>MNAMANKYPTEQLKLWGKAKELREQYYMNYARAKEKGGIRWSGSAWALDAIPAGLGEDVYSLTGEPYAAAVAHDRKFAKECMDAAEAYGFARDLCSYMRIYWGGMHLNKYAFGGEFPKPDFVFQTQICCSHSKWYQHVAKEEKIPEFYLDVGVGPYRDMTDARLDYVANQLHDGIAFVEKASGRKFDDELFIKAVKNEMRSTSRWADICALNKVKPAPLDEKTMYSLYVLCTLSKSSQWCADFMDELYEEVKDRVARGIAAVPNEAIRLMTDTQPPWSFLKIFRYLETYGAVSIGSLYTFALEGIWEDKPDGSWGGRTLPWDKGIEINDRDTAVRLYADWNLSKPQWQHFYDPTIKSDMMLRIIKEWQVDGVMLHLNRGCEGLSVGIMENRLAIAKSGTPVMTFEGNMGDEREFDEVRTQARVDAFMEQLGVRRQAASAWSHPQFEK[2x];>[2x]MSDGLFDQFKTWYEKRHDYARDWKVRTGGQVVATMCTYTPEELLIAAGMLPVRVLGAHEPQNVTEPHIFGMFCPFCRDSLAQGLLGRFDYAEGVTLTQSCIQYRQTFGSWRLHVPTVKWDYYVPMPNEVQSPHARKAHYEEVQAFRVFLQTLTGKEITDAMLSDALAVCDENRRLLRELYEYRKAADPKVTGVEALYASLTAQFIDKREHNEMLKKTLAALPNRKVERKTGARFMTIGSENDDIAFMGMVESVGATIVIDDQCSGSRYFWNASKPEGDVIKAIAERYCDRPACPTKDYPAHTRFDHVLGMAKEYNVEGAIFLQQKFCDPHEGDYPDLKRHLEENGIPTLFLEFDITNPIGPFRIRIEAFLETLSEEELF

An alternative to the classical Birch reduction is provided by dearomatizing benzoyl-coenzyme A (BzCoA) reductases (BCRs) from anaerobic bacteria. BCRs reduce their substrate to cyclohexa-1,5-diene-1-carbonyl-CoA (dienoyl-CoA), representing an ortho- rather than the para-dihydro addition of classical Birch reductions. Architecturally, the heterotetrameric enzyme complexes are composed of two functional dimers: the ATP-binding dimer coordinates a subunit-bridging [4Fe-4S] cluster and serves as an ATP-dependent electron activator, whereas the catalytic dimer is predicted to contain an FeS cluster in each subunit and the substrate binding site. In this study, we heterologously produced the active site components BzdNO from Aromatoleum sp. CIB and provide a first X-ray structural characterization of the catalytic dimer of a class I BCR with the BzCoA substrate and the dienoyl-CoA product in van der Waals contact with the catalytic FeS cluster.

The structure of BzdNO in complex with the product dienoyl-CoA reveals the identical binding mode as the substrate in the BzdNO-BzCoA complex. The dearomatized ring of dienoyl-CoA remains nearly planar; only the C4 sits slightly outside the plane. Instead, it catalyzed the reverse reaction, the methyl viologen-dependent rearomatization of dienoyl-CoA to BzCoA.>[4x]MKVLVTGFEPFGGEKINPTERIAKDLDGIKIGDAQVFGRVLPVVFGKAKEVLEKTLEEIKPDIAIHVGLAPGRSAIS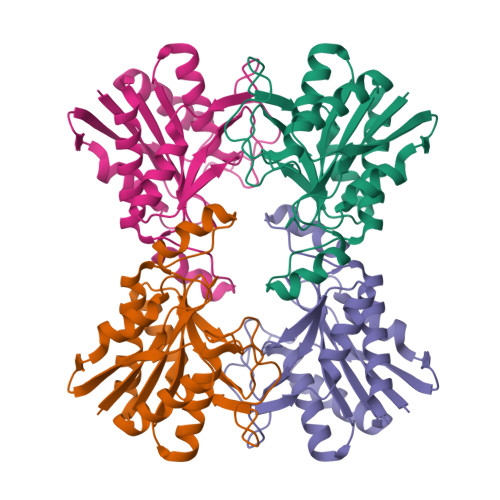IERIAVNAIDARIPDNEGKKIEDEPIVPGAPTAYFSTLPIKKIMKKLHERGIPAYISNSAGLYLSNYVMYLSLHHSATKGYPKMSGFIHVPYIPEQIIDKIGKGQVPPSMSYEMILEAVKVAIEVALEELL>[2x]MVGNRYRLGRKIGSGSFGDIYLGTDIAAGEEVAIKLECVKTKHPQLHIESKIYKMMQGGVGIPTIRWCGAEGDYNVMVMELLGPSLEDLFNFCSRKFSLKTVLLLADQMISRIEYIHSKNFIHRDVKPDNFLMGLGKKGNLVYIIDFGLAKKYRDARTHQHIPYRENK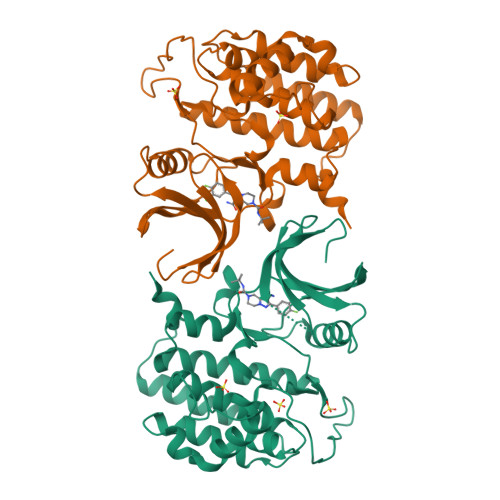NLTGTARYASINTHLGIEQSRRDDLESLGYVLMYFNLGSLPWQGLKAATKRQKYERISEKKMSTPIEVLCKGYPSEFATYLNFCRSLRFDDKPDYSYLRQLFRNLFHRQGFSYDYVFDWNMLK> GVEEIFASGTWHVVDFYGKA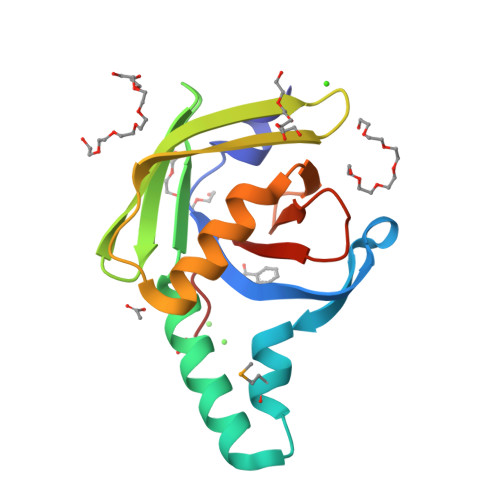NWDKRNGEPKYNAMAHNPDKTIATEGRKALDIIHGFNITFKADGTFTGSIQNGTIEGTWQADGKDRTVNINFTKTPPSTSYNNEFIEALNNAIFYQGDSNVLLLAPEGKKTYIQFAHNKQD> MDYKDDDDKPNPPSFKSHKQNLFNSNNNQHANSVDSFDLHLDDSFDAALDSLQINNNPEPLSKHNTVGDRESFEMRTVDDLDNFSNHSSDSHRKSSNTDTHPLMYDNRLSQDDNFKFTNIASSPPSSSNNIFSKALSYLKVSNTKNWSKFGSPIELSDQHIEREIHPDTTPVYDRNRYVSNELSNAKYNAVTFVPTLLYEQFKFFYNLYFLVVALSQAVPALRIGYLSSYIVPLAFVLTVTMAKEAIDDIQRRRRDRESNNELYHVITRNRSIPSKDLKVGDLIKVHKGDRIPADLVLLQSSEPSGESFIKTDQLDGETDWKLRVACPLTQNLSENDLINRISITASAPEKSIHKFLGKVTYKDSTSNPLSVDNTLWANTVLASSGFCIACVVYTGRDTRQAMNTTTAKVKTGLLELEINSISKILCACVFALSILLVAFAGFHNDDWYIDILRYLILFSTIIPVSLRVNLDLAKSVYAHQIEHDKTIPETIVRTSTIPEDLGRIEYLLSDKTGTLTQNDMQLKKIHLGTVSYTSETLDIVSDYVQSLVSSKNDSLNNSKVALSTTRKDMSFRVRDMILTLAICHNVTPTFEDDELTYQAASPDEIAIVKFTESVGLSLFKRDRHSISLLHEHSGKTLNYEILQVFPFNSDSKRMGIIVRDEQLDEYWFMQKGADTVMSKIVESNDWLEEETGNMAREGLRTLVIGRKKLNKKIYEQFQKEYNDASLSMLNRDQQMSQVITKYLEHDLELLGLTGVEDKLQKDVKSSIELLRNAGIKIWMLTGDKVETARCVSISAKLISRGQYVHTITKVTRPEGAFNQLEYLKINRNACLLIDGESLGMFLKHYEQEFFDVVVHLPTVIACRCTPQQKADVALVIRKMTGKRVCCIGDGGNDVSMIQCADVGVGIVGKEGKQASLAADFSITQFCHLTELLLWHGRNSYKRSAKLAQFVMHRGLIIAICQAVYSICSLFEPIALYQGWLMVGYATCYTMAPVFSLTLDHDIEESLTKIYPELYKELTEGKSLSYKTFFVWVLLSLFQGSVIQLFSQAFTSLLDTDFTRMVAISFTALVVNELIMVALEIYTWNKTMLVTEIATLLFYIVSVPFLGDYFDLGYMTTVNYYAGLLVILLISIFPVWTAKAIYRRLHPPSYAKVQEFATP

In budding yeast, NEO1 is required for neomycin resistance and encodes a phospholipid flippase that establishes membrane asymmetry. Neo1 and Drs2 are Golgi-localized PS/PE flippases, orthologous to human ATP9A/B and ATP8A1/2, respectively, required to establish plasma membrane PS/PE asymmetry. In cells deficient for Neo1/ATP9A, the extracellular PI4P is a receptor that concentrates neomycin on the cell surface and facilitates cellular entry of this aminoglycoside antibiotic. In addition to the previously described PS and PE flippase activity, Neo1/ATP9A also functions as a PI4P flippase, transporting PI4P from the lumenal leaflet of the Golgi to the cytosolic leaflet. Here, we describe a mechanism by which the P4-ATPase Neo1 in budding yeast and the orthologous ATP9A in human cells confer neomycin resistance by preventing PI4P secretion to the extracellular leaflet of the plasma membrane.

The cryo-EM structure of Neo1 in the E2P state with bound PI4P provides further insight into substrate selection and transport mechanisms by P4-ATPases. We observed a lipid-like EM density that fits well with a modelled PI4P. PI4P is at the substrate exit site, representing a post-flipping PI4P in Neo1. Interestingly, the lipid entry site is closed, similar to the closed entry site observed in the Neo1 E2P structure previously determined in detergents. The headgroup of PI4P resides in a large cavity next to TM4, with the terminal phosphate forming hydrogen bonds with a pair of histidine residues (His472 and His476) (Neo1-PI4P). Glu475 forms two hydrogen bonds with the PI4P headgroup to stabilize the substrate further. PI4P binds in the same exit site position and orientation observed for substrate lipid bound in the Dnf1-Lem3 flippase. Thus, the PI4P binding site in Neo1 is within the substrate translocation pathway and is on the opposite side of the membrane domain relative to the PI4P binding site in Drs2. By contrast, the PI4P binding is weaker in Neo1, perhaps evolved for facile substrate release into the membrane. Consistent with a flippase–substrate interaction, the neo1-H472A E475A double mutant causes a loss of PI4P asymmetry and hypersensitivity to neomycin.> MKEEVVIPTTAPRTVLIYFAGDNSLSGYVSQNLRAIKEGIERDGLNNGNLLIYTDKQNEAPQLFQLKLEADTIRQIVLETYASNQNSASTETLTQIIDKVQKEYPADSY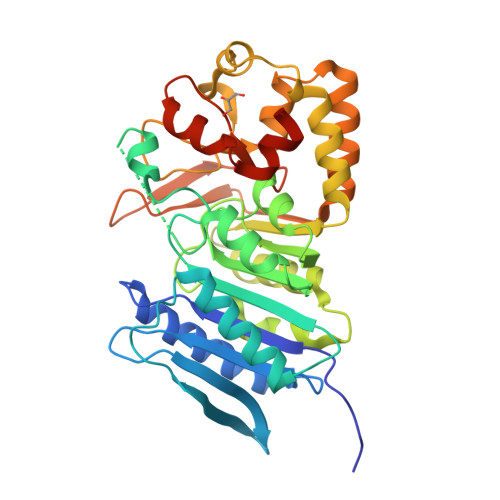GLVLWSHGTGWLPSDIYSYLRSFGQDGKNNFMEINDLASALSKYHFDFILFDACYMSCAEVAYAFRGCADYIIGSPTEILANGFPYQTIMGDMFKKEADVVGIATKFYTYYQSEAGTISVMKSDELDELAATCRTLFHDKTESDLFAVPVSELQIMEYLTPNYHALYDFDDYVSRLATEEQYNAFKRSMEKAVIYKATTPKAVYAYPYPYGSYLPVNKYSGLSIYVPQEALPKLNEWYKDLEWYKDVYQAAALEHHHHHH1,2-DILINOLEOYL-SN-GLYCERO-3-PHOSPHOCHOLINE | C44 H80 N O8 P | 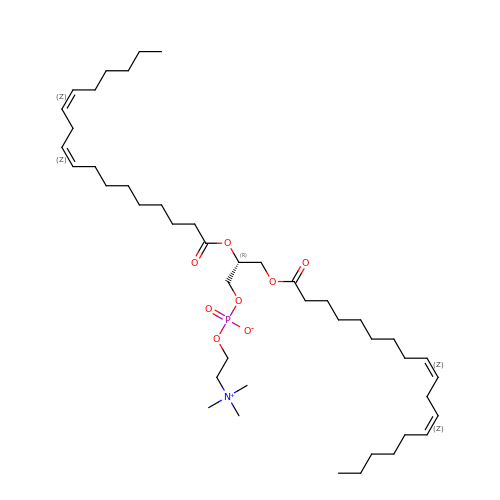FVXDQWZBHIXIEJ-LNDKUQBDSA-N>[4x]GAMDYSLVKALQTAQQNFVISDPSIPDNPIVYASQGFLTLTGYALSEVLGRNCRFLQ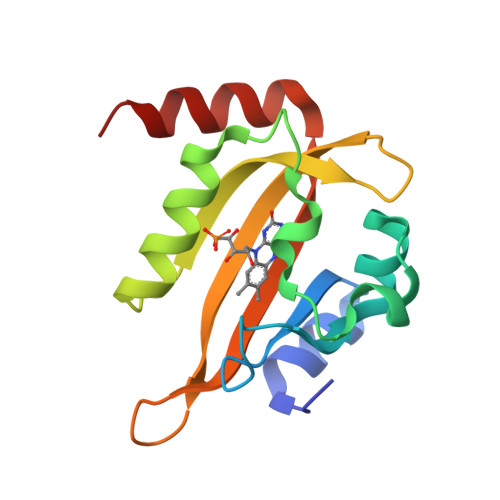GPETDPKAVEKVRKGLERGEDTTVVLLNYRKDGSTFWNQLFIAALRDGEGNVVNYLGVQCKVSEDYAKAFLKNEENE>VQPFAWQVASLADRYEESFDIGAAVEPHQLNGRQGKVLKHHYNSIVAENAMKPISLQPEEGVFTWDGADAIVEF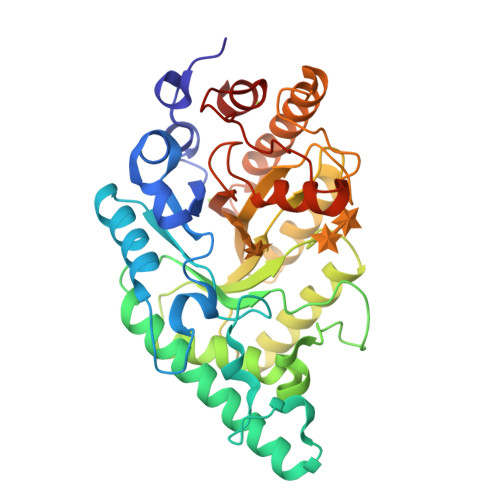ARKNNMNLRFHTLVWHNQVPDWFFLDEEGNPMVEETNEAKRQANKELLLERLETHIKTVVERYKDDVTAWDVVNEVVDDGTPNERGLRESVWYQITGDEYIRVAFETARKYAGEDAKLFINDYNTEVTPKRDHLYNLVQDLLADGVPIDGVGHQAHIQIDWPTIDEIRTSMEMFAGLGLDNQVTELDVSLYGWPPRPAFPTYDAIPQERFQAQADRYNQLFELYEELDADLSSVTFWGIADNHTWLDDRAREYNDGVGKDAPFVFDPNYRVKPAFWRIID[2x]> MSDIVYMGNKALYLILIFSLWPVGIATVIGLSIGLLQTVTQLQEQTLPFGIKLIGVSISLLLLSG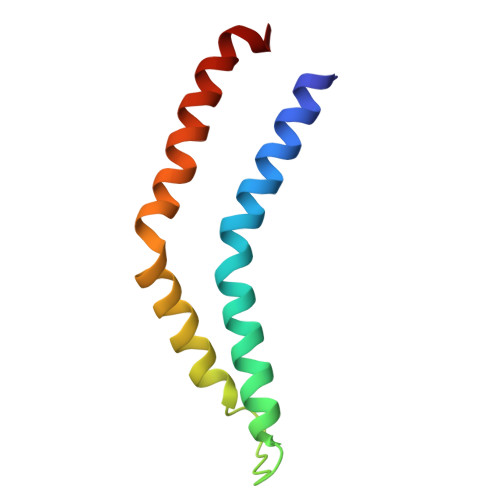WYGEVLLSFCHEIMFLIKSGV>SGTTNTVAAYNLTWKSTNFKTILEWEPKPVNQVYTVQISTKSGDWKSKCFYTTDTECDL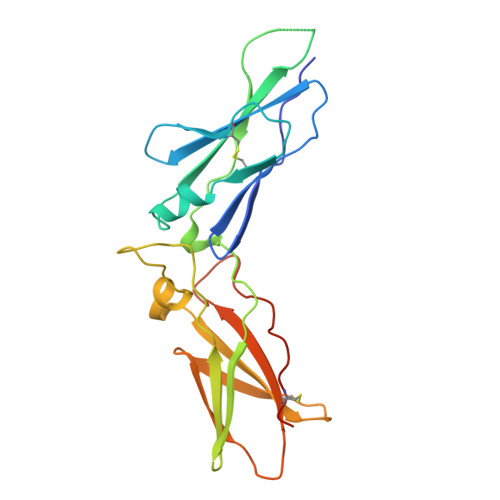TDEIVKDVKQTYLARVFSYPAGNVESTGSAGEPLYENSPEFTPYLETNLGQPTIQSFEQVGTKVNVTVEDERTLVRRNNTFLSLRDVFGKDLIYTLYYWKSSSSGKKTAKTNTNEFLIDVDKGENYCFSVQAVIPSRTVNRKSTDSPVECMGQEKGEFRE[2x]(2R)-oxiran-2-ylmethyl beta-D-xylopyranoside 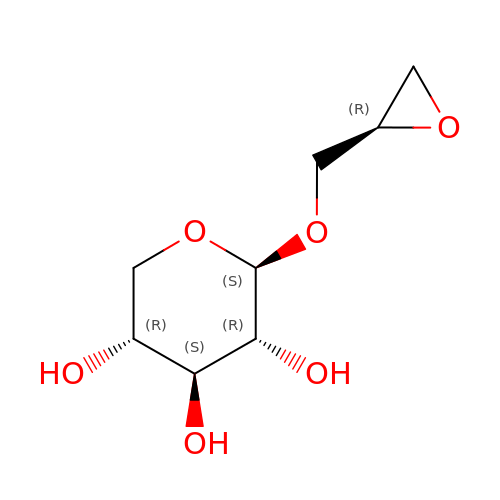| C8 H14 O6 | JKWGJZWJCPSTJC-JAJWTYFOSA-N> MGHHHHHHLEILQIIKESQQQHGLRHGDFQRYRGYCSRRQRRLRKTLNFKMGNRHKFTGKKVTEDLLTDN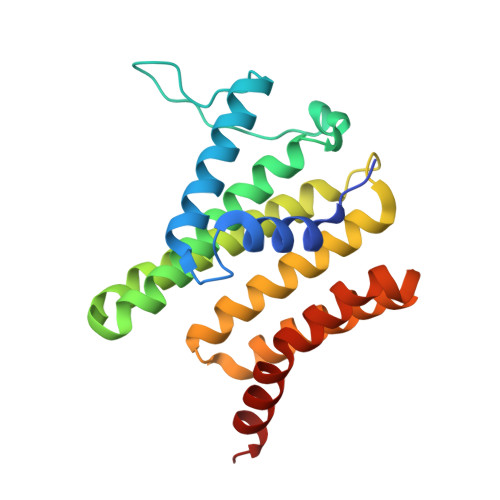RYLLLVLMDAERAWSYAMQLKQEANTEPRKRFHLLSRLRKAVKHAEELERLCESNRVDAKTKLEAQAYTAYLSGMLRFEHQEWKAAIEAFNKCKTIYEKLASAFTEEQAVLYNQRVEEISPNIRYCAYNIGDQ>APNFSSYPFTLGVASGDPLSDSVVLWTRLAPDPLNGGGMPKQAVPVKWEVAKDEHFRKIVRKGTEMAKPSLAHSVHVEADGLEPNKVYYYRFKTGHELSPVGKTKTLPAPGANVPQMTFAFASCQQYEHGYYTAYKHMAKEKLDLVFHLGDYIYEYGPNEYVSKTGNVRTHNSAEIITLQDYRNRHAQYRSDANLKAAHAAFPWVVTWDDHEVENNYANKIPEKGQSVEAFVLRRAAAYQAYYEHMPLRISSLPNGPDMQLYRHFTYGNLASFNVLDTRQYRDDQANNDGNKPPSDESRNPNRTLLGKEQEQWLFNNLGSSTAHWNVLAQQIFFAKWNFGTSASPIYSMDSWDGYPAQRERVINFIKSKNLNNVVVLTGDVHASWASNLHVDFEKTSSKIFGAEFVGTSITSGGNGADKRADTDQILKENPHIQFFNDYRGYVRCTVTPHQWKADYRVMPFVTEPGAAISTRASFVYQKDQTGLRKVSSTTIQGGVKQSDEVEEDRFFSHNK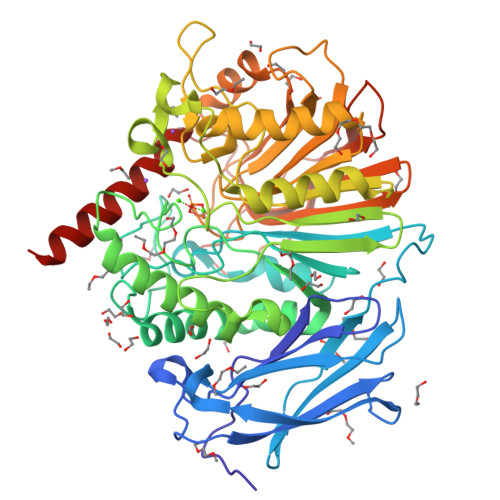AHEKQMIKKRAKITN[2x]Here, we showed three complex structures of 6mA demethylase C. elegans NMAD-1A, a canonical isoform of NMAD-1 (F09F7.7). NMAD-1, one of the AlkB family members in C. elegans, demethylates the DNA damage modification such as 6mA and 3mC. C. elegans NMAD-1A protein has 291 residues involving an N-terminal extension (NTE), a nucleotide-recognition lid (NRL), a DSBH domain, and the CTD. Like other AlkB family proteins, NMAD-1A requires the binding of the cosubstrate α-KG and ferrous iron for catalysis.

At first, we obtained a structure of the WT construct NMAD-1A (residues 21–263) missing the CTD at the resolution of 2.7 Å after extensive screening of protein constructs and crystallization trials. Surprisingly, the active center in this structure was distorted as reflected by the flipping of Asp-186 away from the active site, indicating the importance of the CTD. Additionally, the Met-188 of NMAD-1A took a significant conformational change in the presence of SO42− and was very conserved among sequence alignments of NMAD-1A orthologs. The CTD of NMAD-1A is far away from the active center, however, its loss dramatically compromises the demethylation activity. The CTD-deleted construct NMAD-1A1-263 decreased the demethylation activity sharply. To obtain a structure with a typical active site’s conformation, we used full-length NMAD-1A or certain NMAD-1A constructs containing the CTD for additional crystal screening. However, all experiments to obtain crystals suitable for X-ray diffraction failed.

> GSMTTERVKKLRVVEDKHVNYKVFIYDHIRQIAIPTTNLNSQSSLEDIIDESTSCQSVSTDGSIEIDGLTLIHNFLSESEESKILNMIDTVEWAQSQSGRRKQDYGPKVNFKHKKVKTDTFVGMPEYADMLLNKMSEYDVKKLGNYQPFEMCNLEYEEVKKSAIEMHQDDMWIWGNRLISINLINGSVMTLSNDNKSFLCYVHMPHRSLLCMADECRYDWKHGVLAHHIRGRRIALTMREAAKDFA>[2x]MASGVEDTKHYEEAKKCVEELALYLKPLSSARGVGLNSTTQSVLSRPMQRKLVTLVHCQLVEEEGRIRAMRAARSLGERTVTELILQHQN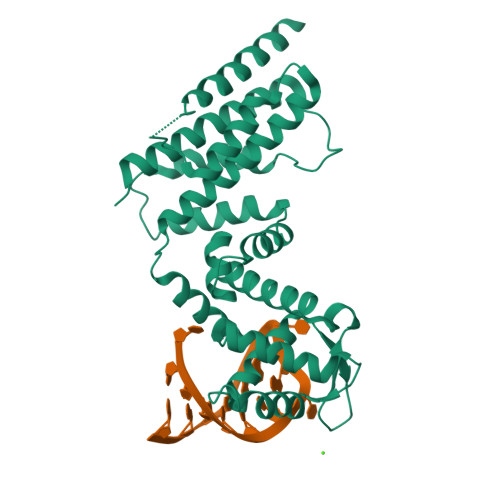PQQLSSNLWAAVRARGCQFLGPAMQEEALKLVLLALEDGSALSRKVLVLFVVQRLEPRFPQASKTSIGHVVQLLYRASCFKVTKRDEDSSLMQLKEEFRTYEALRREHDSQIVQIAMEAGLRIAPDQWSSLLYGDQSHKSHMQSIIDKLQTPASFAQSVQELTIALQRTGDPANLNRLRPHLELLANIDPSPDAPPPTWEQLENGLVAVRTVVHGLVDYIQNHSKKGADQQQLEHHHHHH>[4x]DYLFKVVLIGDSGVGKSNLLSRFTRNEFNLESKSTIGVEFATRSIQVDGKTIKAQI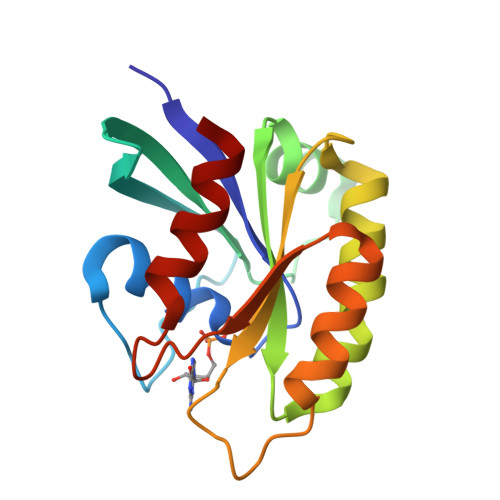WDTAGQERYRAITSAYYRGAVGALLVYDIAKHLTYENVERWLKELRDHADSNIVIMLVGNKSDLRHLRAVPTDEARAFAEKNGLSFIETSALDSTNVEAAFQTILTEIY;> EYDYLFKVVLIGDSGVGKSNLLSRFTRNEFNLESKSTIGVEFATRSIQVDGKTIKAQIWDTAGQERYRAITSAYYRGAVGALLVYDIAKHLTYENVERWLKELRDHADSNIVIMLVGNKSDLRHLRAVPTDEARAFAEKNGLSFIETSALDSTNVEAAFQTILTEIY;> DEYDYLFKVVLIGDSGVGKSNLLSRFTRNEFNLESKSTIGVEFATRSIQVDGKTIKAQIWDTAGQERYRAITSAYYRGAVGALLVYDIAKHLTYENVERWLKELRDHADSNIVIMLVGNKSDLRHLRAVPTDEARAFAEKNGLSFIETSALDSTNVEAAFQTILTEIY> CAGAGCCTGACATACCGCA;> TGC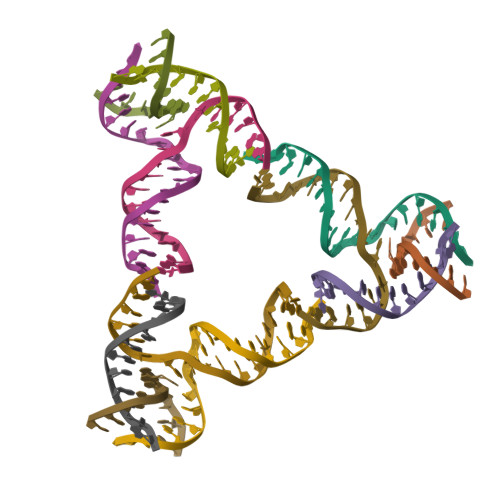GGTATGTCACCACGA;> TGCGCTGTGGCTC;> TCGTGGACAGCG> MSVPTDGAVTTSQIPASEQETLVRPKPLLLKLLKSVGAQKDTYTMKEVLFYLGQYI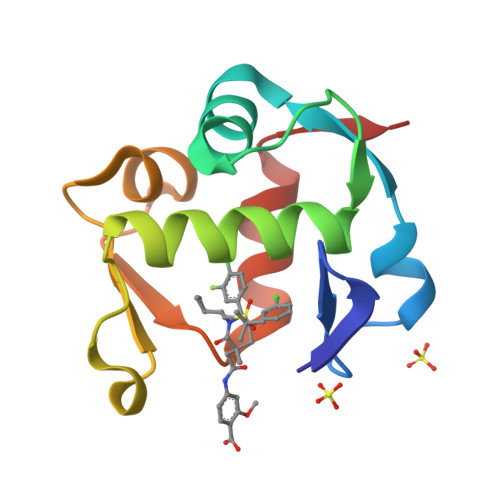MTKRLYDEKQQHIVYCSNDLLGDLFGVPSFSVKEHRKIYTMIYRNLVVV>MSIRTVGIVGAGTMGNGIAQACAVVGLNVVMVDISDAAVQKGVATVASSLDRLIKKEKLTEADKASALARIKGSTSYDDLKATDIVIEAATENYDLKVKILKQIDGIVGE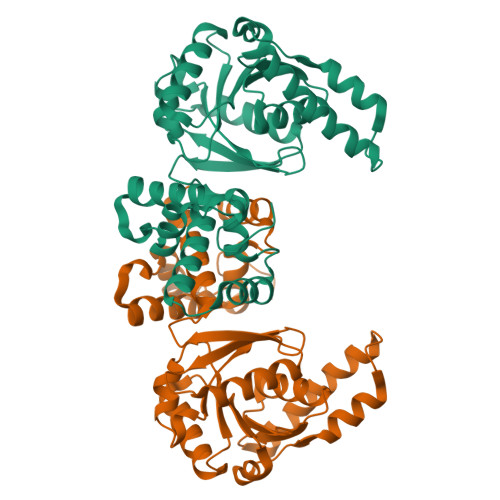NVIIASNTSSISITKLAAVTSRADRFIGMHFFNPVPVMALVELIRGLQTSDTTHAAVEALSKQLGKYPITVKNSPGFVVNRILCPMINEAFCVLGEGLASPEEIDEGMKLGCNHPIGPLALADMIGLDTMLAVMEVLYTEFADPKYRPAMLMREMVAAGYLGRKTGRGVYVYSK[3x]> MVQSMTSVVKAANFILARPTLSKIITPLAQKFTAYAGYREMGLKFNDLLLEETPIMQTAIKRLPSELNYSRNFRILTAHQLALSHQLLPAEKAVKPEEDDNYLIPYILEAEKEAFEKAEL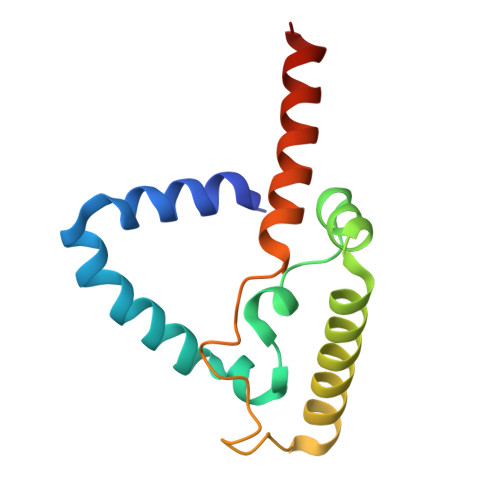DNIEVKA> SMEMNSVMHNDLKEVLLTEEDIQNICKELGAQLTKDYQGKPLVCVGILKGSAMFMSDLIKRIDTHLSIDFMDVSSYHGGTESTGEVQIIKDLGSSIENKDVLIIEDILETGTTLKSITE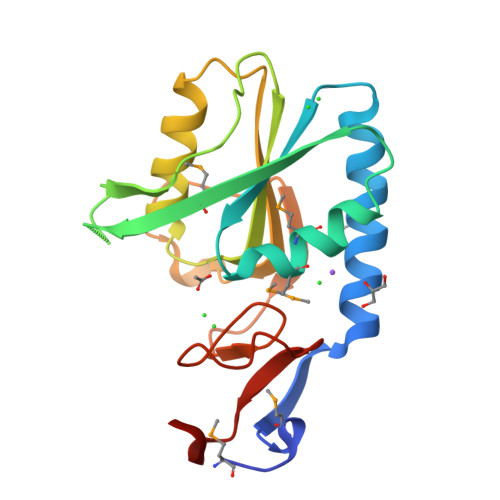LLQSRKVNSLEIVTLLDKPNRRKADIEAKYVGKKIPDEFVVGYGLDYRELYRNLPYIGTLKPEVYSN> ADKLFINALKKKFEESPEEKKTTFYTLGGWKQSERKTEFVNAGKEVAAKRGIPQYNPDIGTPLGQRVLMPYQVSTTDTYVEGDDLHFVNNAAMQQMWDDIRRTVIVGLNHAHAVIEKRLGKEVTPETITHYLETVNHAMPGAAVVQEHMVETHPALVADSYVKVFTGNDEIADEIDPAFVIDINKQFPEDQAETLKAEVGDGIWQVVRIPTIVSRTCDGATTSRWSAMQIGMSMISAYKQAAGEAATGDFAYAAKHAEVIHMGTYLPVRRARGENEPGGVPFGYLADICQSSRVNYEDPVRVSLDVVATGAMLYDQ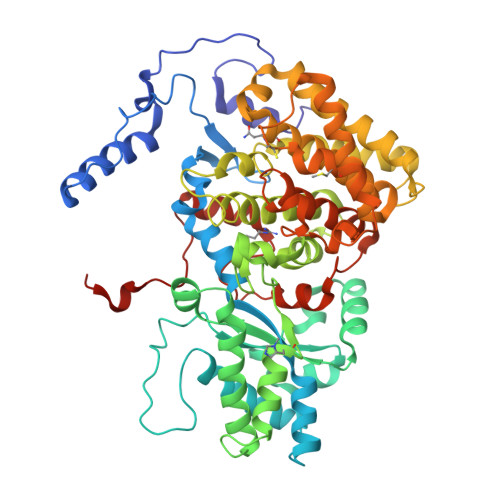IWLGSYMSGGVGFTQYATAAYTDNILDDFTYFGKEYVEDKYGLCEAPNNMDTVLDVATEVTFYGLEQYEEYPALLEDQFGGSQRAAVVAAAAGCSTAFATGNAQTGLSGWYLSMYLHKEQHSRLGFYGYDLQDQCGASNVFSIRGDEGLPLELRGPNYPNYAMNVGHQGEYAGISQAPHAARGDAFVFNPLVKIAFADDNLVFDFTNVRGEFAKGALREFEPAGERALITPAK>[2x]SPSAQELKEQGNRLFVGRKYPEAAACYGRAITRNPLVAVYYTNRALCYLKMQQHEQALADCRRA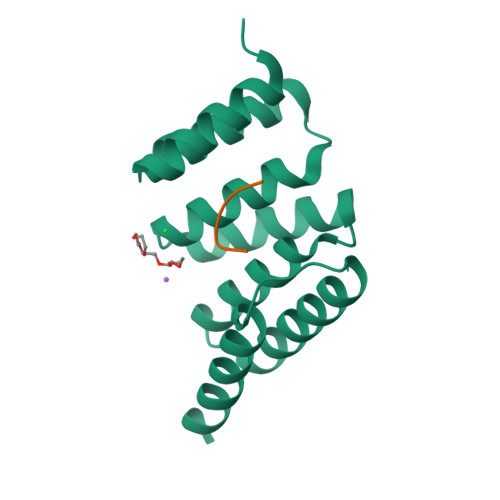LELDGQSVKAHFFLGQCQLEMESYDEAIANLQRAYSLAKEQRLNFGDDIPSALRIAKKKRWNSIEE;>[2x]XLWWPD>[7x]SMRKKIFKPEELRQALMPTLEALYRQDPESLPFRQPVDPQLL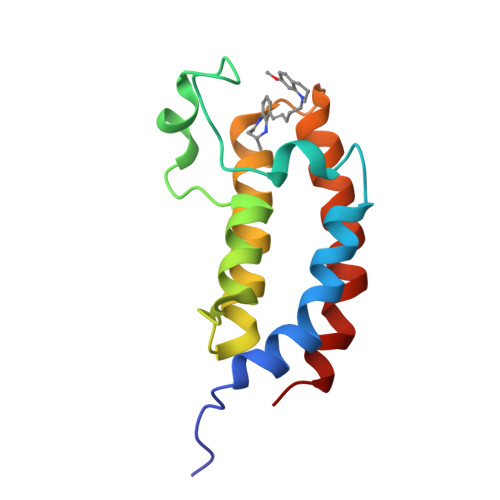GIPDYFDIVKNPMDLSTIKRKLDTGQYQEPWQYVDDVWLMFNNAWLYNRKTSRVYKFCSKLAEVFEQEIDPVMQSLG> GSHMNRLLYAVGGYDGSPDGHTHLNSVECYDPETNEWSLVAPMNTRR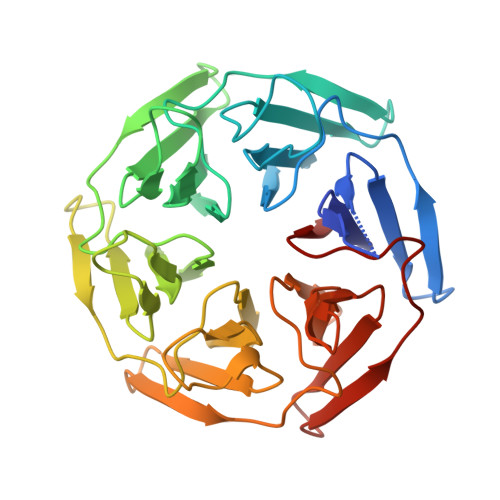SGVGVAVLNRLLYAVGGYDGSPDGHTHLNSVECYDPETNEWSLVAPMNTRRSGVGVAVLNRLLYAVGGYDGSPDGHTHLNSVECYDPETNEWSLVAPMNTRRSGVGVAVLNRLLYAVGGYDGSPDGHTHLNSVECYDPETNEWSLVAPMNTRRSGVGVAVLNRLLYAVGGYDGSPDGHTHLNSVECYDPETNEWSLVAPMNTRRSGVGVAVLNRLLYAVGGYDGSPDGHTHLNSVECYDPETNEWSLVAPMNTRRSGVGVAVL> YAHHPIDYERSTSKSPNILRLPANTSDPTYQENMARMEGLVEQLRARVRYVQAGGVVPEEEAAKAGVSISSIEADDRVRKLHLSRGKMLARDRIERLIDPGTRFLELSQLAGWDLYWDDKKKEYERCYSGGIVTGIGLVNGVRCMLVANDATVKGGTYYPITVKKHLRAQKIAEQNHLPCIYLVDSGGANLSRQDDVFPDEQHFGRIFYNEAQMSIKSISQIAVVMGSCTAGGAYVPAMADENIIVARNGTIFLGGPPLV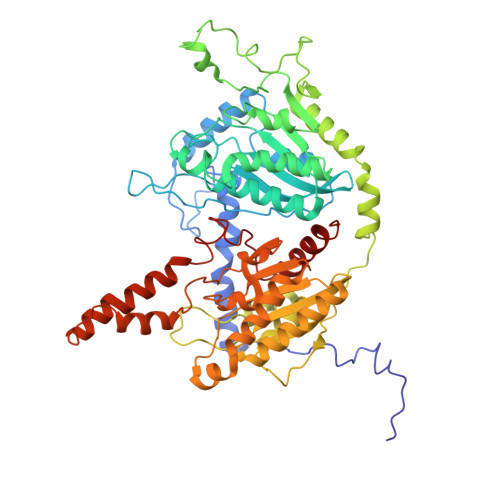LAATGEKVSSEELGGADVHCRISGVGDHYATDDLHALYLARRAVANLNLKEHNEARNPTDVKPVPPLYDPRELGGFIPDMLSDVVKSFDVRAIIARIVDGSRFDEFKALYGNTLVCGFARIEGMQVGIIANQGILYSESALKGAHFIGLCTQRNVPLLFLQNITGFMVGKKYEEGGIARNGARLVMAVSSAPVPKVTVLIGGSYGAGNYGMCGRAFEPRFLFMWPNARISVMGGTQAATVLTLTNRNLKNASEAEIAAFKDKVKKKYEKEGSCYYSTARLWDDGVIAPEDTRVVVAEALRATRLAP> MDEMDNVIRSLEQEYRLILLLNHRNKNQHRAASWYGSFNEMKRNCGQIITLFSSRRLQAKRLKDVEWVKLHRLLQRALF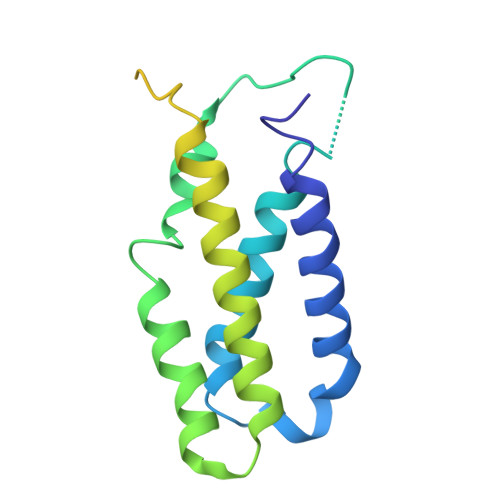RQLKRWYWQFNGVIALGQFVTLGCTLVTLLANVRALYMRLWEINETEFIRCGCLIKNLPRTKAKSVVNDVEELGEIIDEDIGNNVQENELVITSIPKPLTENCKKKKKRKKKNKSAIDGIFG> GMPIPLEKQNKERRQKILTCSLDLFIEKGYYNTSIRDIIALSEVGTGTFYNYFVDKEDILKNLLEDFAKQIISSISEYYLVE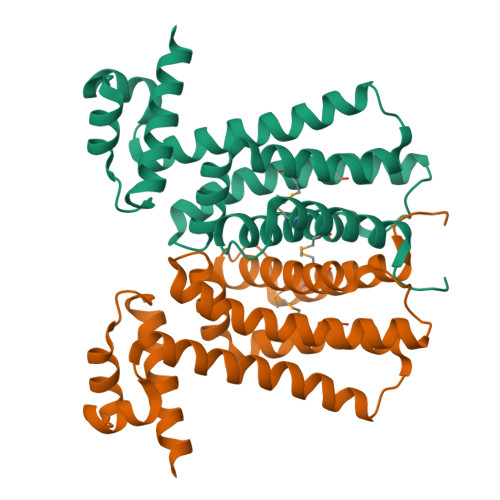KDLYERFIETKRLTMEVFAQNETLSEIYSRVAGSSAPIDQCLKQFEDRLLEFYSRNIEYGIKKGVFKNVPVSPIAHSILAIEKFSLYKWVVLKAITKEEMIEMVLSFHKTLAVGLLVVND N-(3-{[2-(3,4-dihydroxyphenyl)-5,7-dihydroxy-4-oxo-4H-1-benzopyran-3-yl]oxy}propyl)-Nalpha-[(2E)-3-(3,4-dihydroxyphenyl)prop-2-enoyl]-L-tyrosinamide 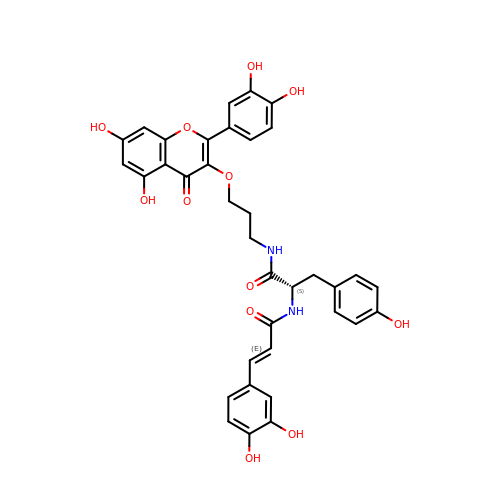| C36 H32 N2 O12 | IRVRXEMGBYHLMY-REHZOHHSSA-N>[3x]MLPAGQDAAALEARQLGGSI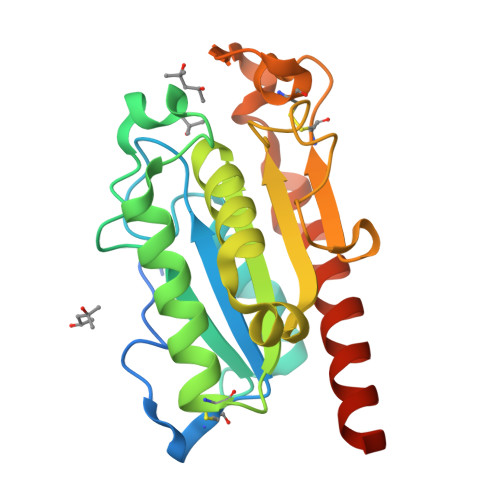TRNDLANGNSGSCPGVIFIYARGSTESGNLGTLGPRVASKLEAKYGKNGVWIQGVGGAYRATLGDNALPRGTSSAAIREMLGHFSDANQKCPDAVLIAGGYSQGAALAAASVTDVDAGIREKIAGAVLFGYTKNLQNRGKIPSYPEDRTKVFCNTGDLVCTGSLIVAAPHLAYQSAASGAAPEFLIQKADAAGAAAAALEHHHHHH>[2x]MAKNDIWTPLESNPDSLYLYSCKLGQSKLKFVDIYGFNNDLLDMIPQPVQAVIFLYPVNDNIVSENNTNDKHNL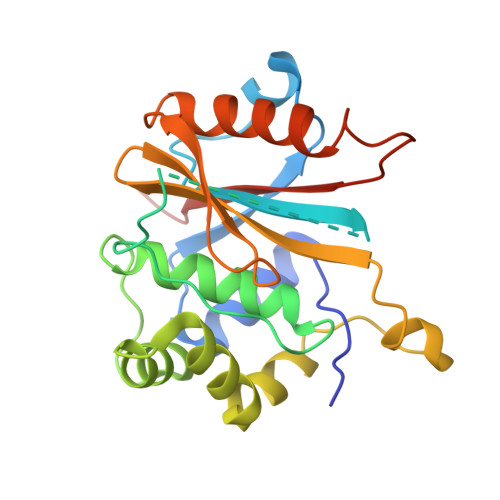KENFDNVWFIKQYIPNSCGTIALLHLYGNLRNKFELDKDSVLDDFFNKVNEMSAEKRGQELKNNKSIENLHHEFCGQVENRDDILDVDTHFIVFVQIEGKIIELDGRKDHPTVHCFTNGDNFLYDTGKIIQDKFIEKCKDDLRFSALAVIPNDNFDII>MPLDAGGQNSTQMVLAPGASIFRCRQCGQTISRRDWLLPMGGDHEHVVFNPHGYIHRVWCFSLAQGLNLIGRPSGEFSWFKGYDWTVAQCGQCGSHLGWHYEGGSQPQTFFGLIKD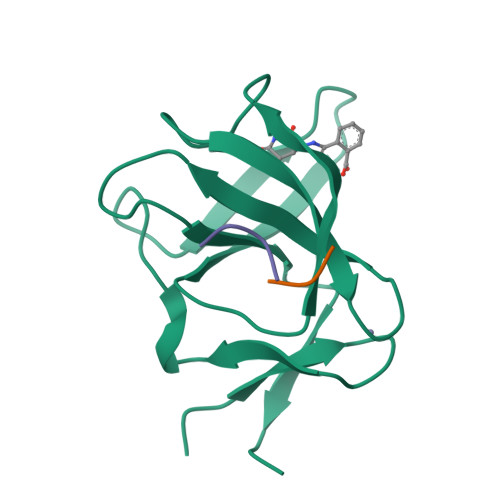RLAEGPAD[4x]> MSSESTTFIVDVSPSMMKNNNVSKSMAYLEYTLLNKSKKSRKTDWISCYLANCPVSENSQEIPNVFQIQSFLAPVTTTATIGFIKRLKQYCDQHSHDSSNEGLQSMIQCLLVVSLDIKQQFQARKILKQIVVFTDNLDDLDITDEEIDLLTEELSTRIILIDCGKDTQEERKKSNWLKLVEAIPNSRIYNMNELLVEITSPATSVVKPVRVFSGELRLGADILSTQTSNPSGSMQDENCLCIKVEAFPATKAVSGLNRKTAVEVEDSQKKERYVGVKSIIEYEIHNEGNKKNVSEDDQSGSSYIPVTISKDSVTKAYRYGADYVVLPSVLVDQTVYESFPGLDLRGFLNREALPRYFLTSESSFITADTRLGCQSDLMAFSALVDVMLENRKIAVARYVSKKDSEVNMCALCPVLIEHSNINSEKKFVKSLTLCRLPFAEDERVTDFPKLLDRTTTSGVPLKKETDGHQIDELMEQFVDSMDTDELPEIPLGNYYQPIGEVTTDTTLPLPSLNKDQEENKKDPLRIPTVFVYRQQQ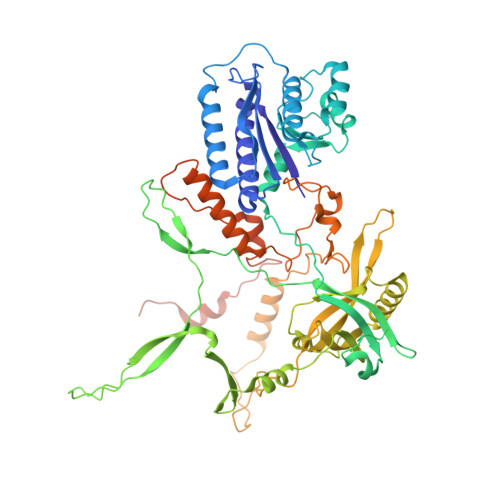VLLEWIHQLMINDSREFEIPELPDSLKNKISPYTHKKFDSTKLVEVLGIKKVDKLKLDSELKTELEREKIPDLETLLKRGEQHSRGSPNNSNN> MQASDEYPGNFKITSHNVYLFSRNIYPNWG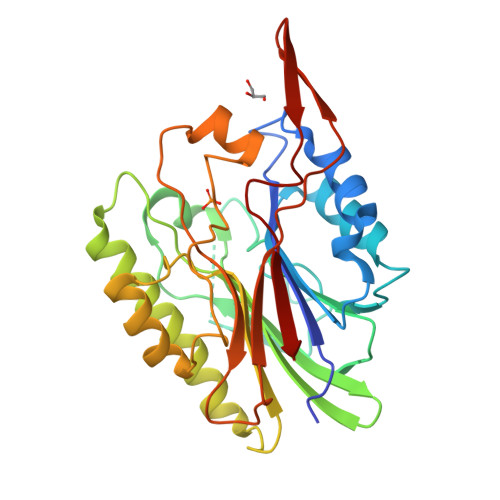QMHRADLIAQADYMKNNDVVILNEAFDTSASHRLLNNLREMYPHQTPVIGRSKHGWDKTEGNYSNFALEDGGVAVVSQWPIVEKSQHIFQRGGGADRLSNKGFAYVKIMKNGKPYHIIGTHTQADDSLISKDTSRAIRAEQMQEIQTFIAKKNIPKDEIIFIGGDLNVNYGTDEYHDMLKLLNVSSPANFNGQMATWDPTTNSMLKESYPKAAPEYLDYIFVENGHARPHSWHNKVLHTKSPQWSVKSWFKTYTYQDFSDHYPVVGFTDNN> FMVSLPRMVYPQPKVLTPCRKDVLVVTPWLAPIVWEGTFN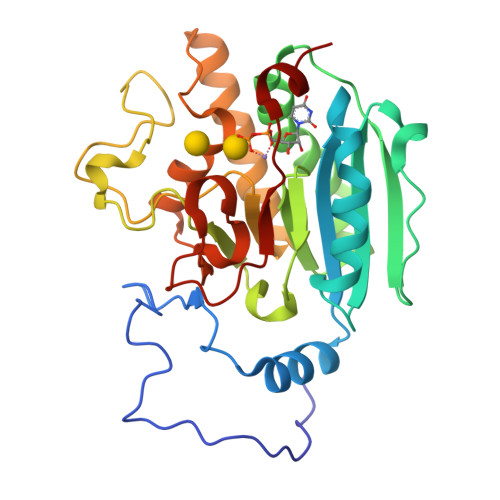IDILNEQFRLQNTTIGLTVFAIKKYVAFLKLFLETAEKHFMVGHRVHYYVFTDQPAAVPRVTLGTGRQLSVLEVRAYKRWQDVSMRRMEMISDFCERRFLSEVDYLVCVDVDMEFRDHVGVEILTPLFGTLHPGFYGSSREAFTYERRPQSQAYIPKDEGDFYYLGGFFGGSVQEVQRLTRACHQAMMVDQANGIEAVWHDESHLNKYLLRHKPTKVLSPEYLWDQQLLGWPAVLRKLRFTAVPKNHQAVRNP Currently, no effective therapies exist for fibrodysplasia ossificans progressiva (FOP), a rare congenital syndrome in which heterotopic bone is formed in soft tissues owing to dysregulated activity of the bone morphogenetic protein (BMP) receptor kinase ALK2 (also known as ACVR1). All cases arise from an autosomal dominant germline mutation in the gene ACVR1 encoding the type I bone morphogenetic protein (BMP) receptor kinase ALK2 (11). Approximately 97% of patients with the classic FOP phenotype harbor the recurrent gain-of-function mutation R206H (c.617G>A). This substitution alters the structure of the receptor’s intracellular domain causing aberrant kinase activation and SMAD1/5/8 phosphorylation in response to activin A as well as hypersensitivity to BMP ligands. The BMP/TGF-β receptors form the only family of serine/threonine transmembrane receptor kinases but map favorably for drug repositioning to the tyrosine kinase-like branch of the human kinome.

Saracatinib is a potent inhibitor of the protein kinase ALK2. Saracatinib binds inactive ALK2 in an αC-in conformation. Within the ATP-binding pocket, the bound ligand was well resolved by the electron density map. Although the quinazoline of saracatinib formed a hydrogen bond to the hinge residue His286, specificity was likely derived from the large chlorobenzodioxole moiety, which nicely complemented the size, shape, and hydrophobicity of the back pocket. The tetrahydropyran ring was located in the ribose pocket below the glycine-rich loop (β1-β2), whereas the methylpiperazine moiety was extended largely into solvent. By contrast, the ALK2 complex exhibited an inactive conformation in which the αC helix was swung inwards to compress the ATP pocket. As a result, the equivalent αC (Glu248) and glycine-rich loop (Tyr219) residues were packed inside the ATP pocket where they mediated additional interaction with the chlorobenzodioxole and tetrahydropyran groups, respectively. Structural differences between the ALK2 and SRC complexes with saracatinib were evident from the different conformations of their catalytic domains. The previously determined SRC complex structure displayed an inactive αC-out conformation that widened the ATP pocket and rotated the αC residue Glu310 away to solvent, as well as the glycine-rich loop residue Phe278. Thus, further optimization of this chemotype could yield molecules with increased selectivity for ALK2 over SRC family kinases.

>SMQRTVARDITLLECVGKGRYGEVWRGSWQGENVAVKIFSSRDEKSWFRETELYNTVMLRHENILGFIASDMTSRHSSTQLWLITHYHEMGSLYDYLQLTTLDTVSCLRIVLSIASGLAHLHIEIFGTQGKPAIAHRDLKSKNILVKKNGQCCIADLGLAVMHSQSTNQLDVGNNPRVGTKRYMAPEVLDETIQVDCFDSYKRVDIWAFGLVLWEVARRMVSNGIVEDYKPPFYDVVPNDPSFEDMRKVVCVDQQRPNIPNRWFSDPTLTSLAKLMKECWYQNPSARLTALRIKKTLTKID[4x]> GKTNDWLDFDQLAEEKVRDALKPPSMYKVILVNDDYTPMEFVIDVLQKFFSYDVERATQLMLAVHYQGKAICGVFTAEVAETKVAMVNKYARENEHPLLCTLEKA;> LVKSK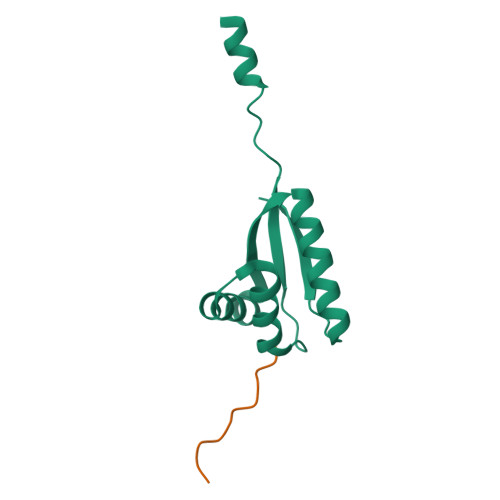ATNLLY> VTSIK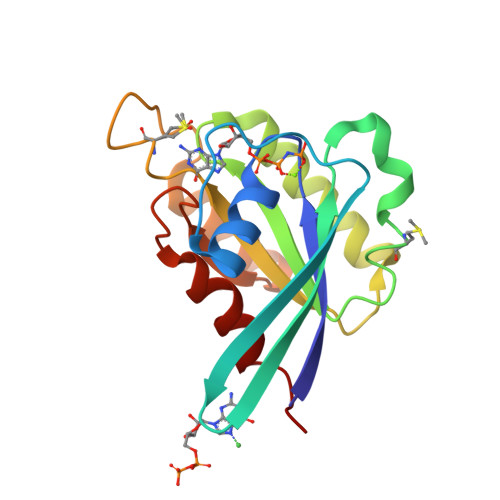LVLLGEAAVGKSSIVLRFVSNDFAENKEPTIGAAFLTQRVTINEHTVKFEIWDTAGQERFASLAPMYYRNAQAALVVYDVTKPQSFIKARHWVKELHEQASKDIIIALVGNKIDMLQEGGERKVAREEGEKLAEEKGLLFFETSAKTGENVNDVFLGIGEKIPLK>HMSSLQRASVSFNKPGHIPFGAVQGYAPGGVPAYSNKHDHYFSGERNIEDNIFFGFKYQCVEFARRWLLVRKGLLLPDVNWACHIFQLKEVRDAATTESFAVLQVRNGTTTKPEADALLVYPSTDANPVGHVGTITEVGDDYVCVADQNYRFHKWESSCAYKLKLDHRDGIWTIIDDIDADEIEIPLGWLTFPGRANRPEGAPPVALHPSLHFKEPPKPYLLRRNFLPTESKANWLDMNNPAERLFVEEFGMDVSRTRLEEKVVSYYESNHEFHLRCVAYGTQLHAIFMEATAQVIESDEKLRLFAIPEEFWPRIRHSWKYQQTYISGRFDFAFNNETGEVKCFEYNADSASTLLECGLIQQKWAESVGLDKQDTRGSGFAVERNLKMAWANSGATGRVHFCVDEEREEQYTALYCMQA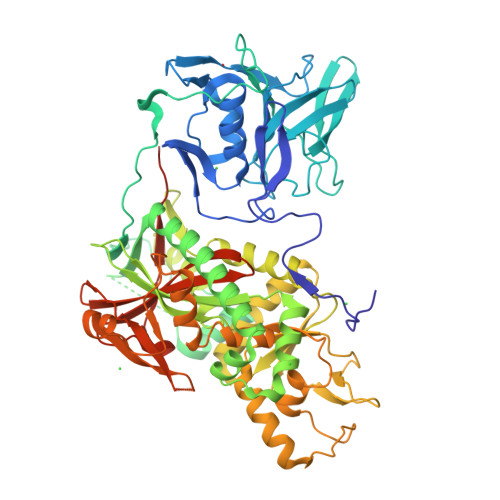AEAVGLEGKLCILFDEFRFDDNGHVVDSDGVRVRNVWKTWMWESAITDYYAAREERGENWKPSPKDKVRLCDLLLGDDWEILYFEPMWKVIPSNKAILPMIYHNHPEHPAILKAEYELTDELRKHGYAKKPIVGRVGSNVIITSGDGVVHAESGGKYGKRNMIYQQLFELKKQDDYYAIIGGWMIGDAFSGTGIREDKSVITGVDSPFAAVRIKTDKLPHPVTLKDIDKMAEDE[2x]CCHFV is classified within the Nairoviridae family of the order Bunyavirales. Its genome comprises three negative sense RNA segments named small (S), medium (M) and large (L), which respectively encode the nucleoprotein (NP), that encapsidates each RNA segment; the glycoprotein precursor, which is post-translationally cleaved to yield envelope glycoproteins Gn and Gc; and the L protein that contains both RNA-dependent RNA polymerase (RdRp) and OTU-like modules, with the latter performing immunomodulatory roles. The RdRp and NP associate with the segments forming ribonucleoproteins (RNPs) that act as templates for all viral RNA synthesis activities. Affimer affinity reagents are a class of non-antibody binding proteins based on a phytocystatin consensus sequence that scaffolds two variable peptide regions that represent target recognition sites. We describe the selection and characterization of a high affinity non-antibody binding protein, Affimer-NP, that specifically recognises the CCHFV nucleocapsid protein (NP).

To further characterize the interaction between Affimer-NP and CCHFV NP and determine the molecular basis for the interference of Affimer-NP with CCHFV NP RNA-binding and gene expression functions, we solved the high-resolution crystal structure of the complex. Two Affimer-NP/CCHFV NP complexes were elucidated per asymmetric unit. The structure shows the variable loops of Affimer-NP bound to the globular domain of CCHFV NP, mainly interacting with the residues Q329, F330, F332, E333, K336, R339, K343, A347, T351, N399, D402 and L405. As previously published structures show, CCHFV NP contains two major domains: a globular core and an extended arm. Although no crystal structure of CCHFV NP in complex with RNA has been solved to date, analysis of its electrostatic surface potential reveals a continuous positively charged region, likely the binding site for RNA, comprising residues R45, K72, S149, H197, K222, R225, K237, Q303, K336, R339, K342, K343, K345, R372, and K462 (highlighted in blue in Fig 4A–4C). CCHFV NP exists as a monomer in the absence of RNA, but different oligomeric forms have been described when bound to RNA of the expression host. The interaction between monomers involves residues 320–354 within the head domain of one molecule and residues 210–219 and 260–272 of the arm of the adjacent molecule (highlighted in pink in Fig 4A–4C). The residues of the globular domain that interact with the variable loops of Affimer-NP all lie between NP residues 320–354, suggesting a potential interference of Affimer-NP in CCHFV NP oligomerization. As both oligomerization and RNA-binding are required for assembly of functional CCHFV RNPs, the location of the Affimer-NP binding site also offers a likely explanation for its ability to disrupt CCHFV mini-genome activity. The specificity of Affimer-NP for CCHFV NP, showing no cross-reactivity with HAZV NP, may also be explained by this crystal structure.

>[2x]MENKIEVNSKDEMNKWFEEFKKGNGLVDTYTNSYSFCESVPNLDRFVFQMAGATDDAQKDSIYASALVEATKFCAPIYECAWASSTGIVKKGLEWFEKNTGTIKSWDESYIELKVEVPKIEQLFNYQQAALKWRKDIGFRVNANTAALSNKVLAEYKVPGEIVMSVKEMLSDMIRRRNLILNRGGDENPRGPVSHEHVEWCREFVKGKYIMAFNPPWGDINKSGRSGIALVATGLAKLAETEGKGVFDEAKKTVEALNGYLDKHKDEVDKASADNMVTNLLKHVAKAQELYKNSSALRAQGAQIDTVFSSYYWLYKAGVTPETFPTVSQFLFELGKHPRGTKKMKKALLSTPMKWGKKLYELFADDSFQQNRIYMHPAVLTAGRISEMGVCFGTIPVANPDDAALGSGHTKSILNLRTNTETNNPCARTIVKLFEIQKTGFNIQDMDIVASEHLLHQSLVGKQSPFQNAYNVKGNATSANII;>[2x]ENSLEIEELARFAVDEHNKKENALLEFVRVVKAKEQMHMKERQINTMYYLTLEAKDGGKKKLYEAKVWVKKYLGDFWKDNFKELQEFKPV Types 1 and P pili are archetypal CU pili produced by uropathogenic Escherichia coli (UPEC) that mediate host-pathogen interactions critical in disease and biofilm formation (Flores-Mireles et al., 2015). Types 1 and P pili are composed of a short tip fibrillum made of three to four different subunits (FimH, FimG, and FimF for type 1 pili and PapG, PapF, PapE, and PapK for P pili) mounted on a 1–2 μM long and helically wound rod, which is composed of ∼1,000 copies of the major pilus subunit FimA or PapA for type 1 or P pili, respectively (Allen et al., 2012, Waksman and Hultgren, 2009). The rod adopts a helical quaternary structure and is thought to play essential roles: its formation may drive pilus extrusion by preventing backsliding of the nascent growing pilus within the secretion pore; the rod also has striking spring-like properties, being able to uncoil and recoil depending on the intensity of shear forces generated by urine flow. During DSE, the donor strand provided by the chaperone to complement the subunit fold is replaced by another subunit’s N-terminal extension (Nte), a 10–20 residue extension found at the N terminus of each subunit except the subunit located at the very tip.

In a crucial step toward being able to test the various putative roles that the pilus rod has in driving translocation and in mediating mechanical resistance to external forces, we solved the 3.8 Å resolution structure of the P pilus rod using cryoelectron microscopy (cryo-EM). P pilus rods were produced in vitro from the purified PapD:PapA complex. The P pilus rod forms a helical filament of 3.28 subunits per turn, a pitch of 25.2 Å, and diameter of ∼81 Å. It contains a continuous central hollow lumen of ∼21 Å in diameter. Strikingly, each subunit makes protein-protein interactions with ten other subunits, five preceding (−5 to −1) and five succeeding (+1 to +5). The subunit-subunit interactions network within the pilus rod is strikingly large, with each subunit burying 45.5% of its total surface area. From residues 1–5, the very N-terminal end of PapA makes extensive stabilizing subunit-subunit contacts. This portion of PapA extends parallel to the rod axis and is termed the “staple” because of the multiple interfaces it makes with other subunits (see below). The sequence after the Nte (from residue 20) forms the pilin fold, a fold previously characterized as a C-terminally truncated Ig-fold-lacking strand G. Compared to the structure of PapA in dimers (representing a state of PapA prior to incorporation in the rod), the structure of PapA in the rod has undergone a substantial conformational change in the region between strands βB and βC, where contacts with an adjacent subunit stabilize an extended region into a three-turn α-helix, αA3.

>APTIPQGQGKVTFNGTVVDAPCSISQKSADQSIDFGQLSKSFLEAGGVSKPMDLDIELVNCDITAFKGGNGAKKGTVKLAFTGPIVNGHSDELDTNGGTGTAIVVQGAGKNVVFDGSEGDANTLKDGENVLHYTAVVKKSSAVGAAVTEGAFSAVANFNLTYQ[13x]> ISEV;> QGIEDLISEVAQGALTLSLPKQQDSLPDTKASGPAHSKEVPALTAVETGATNPLAPSDTVQTRHVVQRRSRSESTIESFFARGACVAIIEVDNEQPTTRAQKLFAMWRITYKDTVQLRRKLEFFTYSRFDMEFTFVVTANFTNANNGHALNQVYQIMYIPPGAPTPKSWDDYTWQTSSNPSIFYTYGAAPARISVPYVGLANAYSHFYDGFAKVPLKTDANDQIGDSLYSAMTVDDFGVLAVRVVNDHNPTKVTSKVRIYMKPKHVRVWCPRPPRAVPYYGPGVDYRNNLDPLSEKGLTTY;> SPNVEACGYSDRVLQLTLGNSTITTQEAANSVVAYGRWPEFIRDDEANPVDQPTEPDVATCRFYTLDTVMWGKESKGWWWKLPDALRDMGLFGQNMYYHYLGRSGYTVHVQCNASKFHQGALGVFAIPEYCLAGDSDKQRYTSYANANPGERGGKFYSQFNKDNAVTSPKREFCPVDYLLGCGVLLGNAFVYPHQIINLRTNNSATIVLPYVNALAIDSMVKHNNWG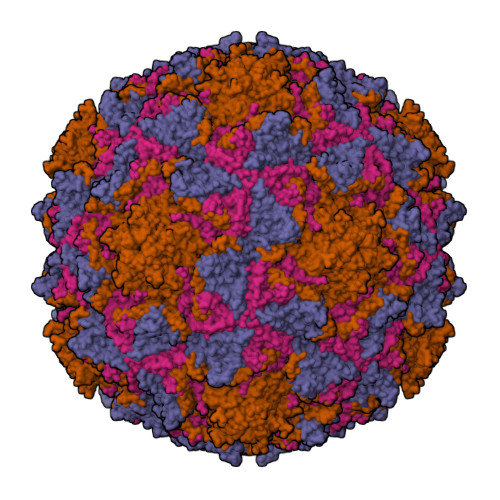IAILPLSPLDFAQDSSVEIPITVTIAPMCSEFNGLRNVTAPKFQ;> GLPVLNTPGSNQYLTSDNHQSPCAIPEFDVTPPIDIPGEVKNMMELAEIDTMIPLNLESTKRNTMDMYRVTLSDSADLSQPILCLSLSPAFDPRLSHTMLGEVLNYYTHWAGSLKFTFLFCGSMMATGKILVAYAPPGAQPPTSRKEAMLGTHVIWDLGLQSSCTMVVPWISNVTYRQTTQDSFTEGGYISMFYQTRIVVPLSTPKSMSMLGFVSACNDFSVRLLRDTTHISQSALPQ;> GAQVSSQKVGAHENSNRAYGGSTINYTTINYYKDSASNAASKQDYSQDPSKFTEPLKDVLIKTAPALN> MASAGVAAGRQAEDVLPPTSDQPLPDTKPLPPPQPPPVPAPQPQQSPAPRPQSPARAREEENYSFLPLVHNIIKCMDKDSPEVHQDLNALKSKFQEMRKLISTMPGIHLSPEQQQQQLQSLREQVRTKNELLQKYKSL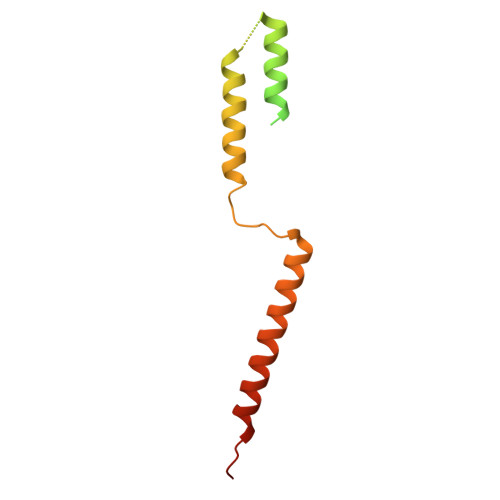CMFEIPKE> MTKLFSKVKESIEGIKMPSTLTINGKAPIVAYAELIAARIVNALAPNSIAIKLVDDKKAPAAKLDDATEDVFNKITSKFAAIFDNGDKEQVAKWVNLAQKELVIKNFAKLSQSLETLDSQLNLRTFILGGLKYSAADVACWGALRSNGMCGSIIKNKVDVNVSRWYTLLEMDPIFGEAHDFLSKSLLELKKSANVGKKKETHKANFE;> MSDLVTKFESLIISKYPVSFTKEQSAQAAQWESVLKSGQIQPHLDQLNLVLRDNTFIVSTLYPTSTDVHVFE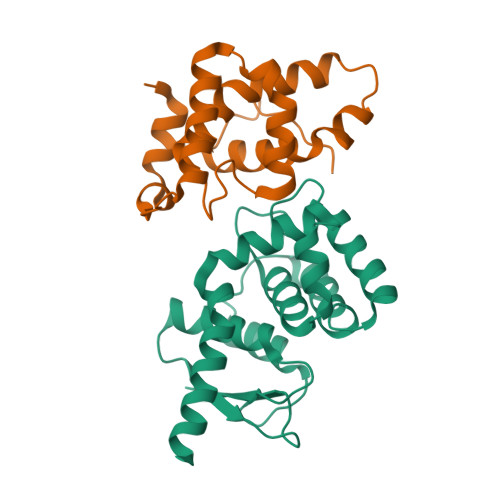VALPLIKDLVASSKDVKSTYTTYRHILRWIDYMQNLLEVSSTDKLEINHD>[4x]GSHMMERPQPDSMPQDLSEALKEATKEVRTQAENAEFMRNFQKGQVTRDGFKLVMASLYHIYVALEEEIERNKESPVFAPVYFPEELHRKAALEQDLAFWYGPRWQEVIPYTPAMQRYVKRLHEVGRTEPELLVAHAYTRYLGDLSGGQVLKKIAQKALDLPSSGEGLAFFTFPNIASATKFKQLYRSRMNSLEMTPAVRQRVIEEAKTAFLLNIQLFEELQELLTHDTKDQSPSRAPGLRQRASNK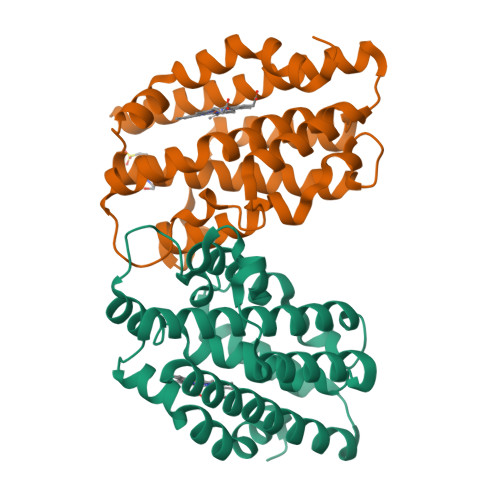VQDSAPVETPRGKPPLNTRSQAPLLRWVLTLSFLVATVAVGLYAM We investigated a TRPM2 chanzyme from choanoflagellates that integrates two seemingly incompatible functions into a single peptide: a channel module activated by ADP-ribose with high open probability and an enzyme module (NUDT9-H domain) consuming ADP-ribose at a remarkably slow rate. Using time-resolved cryogenic-electron microscopy, we captured a complete series of structural snapshots of gating and catalytic cycles, revealing the coupling mechanism between channel gating and enzymatic activity. The slow kinetics of the NUDT9-H enzyme module confers a self-regulatory mechanism: ADPR binding triggers NUDT9-H tetramerization, promoting channel opening, while subsequent hydrolysis reduces local ADPR, inducing channel closure. The structures of srTRPM2 exhibit a characteristic TRPM architecture, from top to bottom, a transmembrane domain (TMD) layer containing the ion-conducting pore, a signal transduction layer consisting of MHR3/4 domain and the C-terminal rib helix, and an ADPR-sensing layer consisting of the N-terminal MHR1/2 domain and the C-terminal NUDT9-H domain.

A cation binding site is found between the MHR3/4 domain and the Rib helix of each subunit, termed MgMHR. This site does not distinguish between Ca2+ or Mg2+ either and is unique to srTRPM2 as the key residue, E1114, is not conserved. Replacing E1114 with alanine eliminated cation binding at MgMHR, resulting in a reduced rotational movement of the intracellular domain around the symmetry axis when ligands were bound, as compared to the wild-type (WT) protein. The E1114A mutation had no obvious effect on macroscopic currents. However, single-channel analysis showed a small decrease in channel open probability and a small increase in channel close rate, revealing a regulatory role of this cation binding site on channel gating.

>[4x]MQRARPGELVEVIMFRPTGKARVSNLDESMAMEFTDLRTRAMSSAAMIRQSVAAKTLLIENEDGKGSTRMEVQDFMKRFHMHASEDDKTGSPSTAWGTLRFPTKEATAPYLRLSVNDDPEDALLFVKAMLAQKYGETYDRPSLILSVTGGARNFTLPPRLETAIAKGLRLAAQRTNAWVVTGGTNTGVMKLTGQIMEALSKTQSHFIPPTIGIATYGVIIGGDDMTRGEPPKIGLEYEMHKKDPPKTTPLDDNHNLFLLVDDGSTNKFGKEIKFRAAFENAAGQAFAAPVVTIVVQGGPGTLGTALQAVRQGTPIVVVDGSGLAADVLAYAYNFMHNPLTRFKSYTIDDLRQKVAQTFNPKSSQQLTNLLDSALECVQDPNLVVVYSLQESGIDEFDDCILKAIFSSQGKLGNKLKQAMYFDQLDVAKRALSEASKNGQHNEIAACINDNLMAAMMHNKPHFVELYLGFDAKIYELKPSEEVAKTNITALDELPSFALAIEELYKREAKKPHSHVQRLVSLSNTDVLGRHYRVSTQRGDGTTRRIGRDLANTRAYNVLRMDQIFARLVSKDFSVNRDFTIYDSKYDKVPGIQFRRTAQASHMLFLWAICLDRFRMARHFWLIGDQSIINALVASRILERLSTHRALQGPHLAEERAKMQHNAKKFEELAVGVLGECHGSDSHMASEMLHSKNDMFNKKNAINIAYDAKSLAFLSHPATQSVINADWYGHLKSVTSFWAVLFAFFFPFFVLPFINFSEDHAEQQVEAPRDFFTDAPRSSHSANSTTSGAHRLRRKFAKFYSAPYTRFISDLLSHFVLCVVTSYFVLDKLEDTISAIEWILLVWFVALLLEELRQMIFCDGIAEYISDTWNRLDLIMITLFFVGFFTHASDPSNQDSKVVSKGIHAFLVVVLWLRFMRYYALSKNLGPKLIMMMEMMKDVSTFVFLLLIFLIGYGVAAQSLLSPDEDFSSRTFIGVLFRPYFQIYGELFLDDLNSEANCLGDTPFTECSRETVRMVPFFLAVYILGSNVLLVNLLIAMFNDTYMKVQEAAEDLWRKQNYELCAEYKDRPFLPAPFILLAHVHMLFMRLLRLCGVHTQEHEKIQDDETKRKITTFEALNTDKFLRRWERERQEMLEARVKMTNDNVVQAMGMMDQLLEHMISFRFSLDQQATKIKQEIRDDGLPSTEPTGLVSRTPSQPINRLNSAVAVHGHTAEAAEWYVPPEEYPKSGGVKRYLIDASMVPLSIMCPSYDPVEYTHPSVAAQPVWADPADPRKIKFNVKDEVNGKVVDRTSCHPSGISIDSNTGRPINPWGRTGMTGRGLLGKWGVNQAADTVVTRWKRSPDGSILERDGKKVLEFVAIQRQDNKMWAIPGGFVDNGEDVALTSGREFMEEALGMGTSADLMSAESKDSLAALFSSGTIVARIYCEDPRNTDNAWVETTCVNFHDESGRHAARLKLQGGDDAEHARWMMVHGGLNLFASHRTLLQHVTSALNAYF>GGAKPLTDQEKRRQISIRGIVGVENVAELKKSFNRHLHFTLVKDRNVATTRDYYFALAHTVRDHLVGRWIRTQQHYYDKCPKRVYYLSLEFYMGRTLQNTMINLGLQNACDEAIYQLGLDIEELEEIEEDAGLGNGGLGRLAACFLDSMATLGLAAYGYGIRYEYGIFNQKIRDGWQVEEADDWLRYGNPWEKSRPEFMLPVHFYGKVEHTNTGTKWIDTQVVLALPYDTPVPGYMNNTVNTMRLWSARAPNDFNLRDFNVGDYIQAVLDRNLAENISRVLYPNDNFFEGKELRLKQEYFVVAATLQDIIRRFKASKFGSTRGAGTVFDAFPDQVAIQLNDTHPALAIPELMRIFVDIEKLPWSKAWELTQKTFAYTNHTVLPEALERWPVDLVEKLLPRHLEIIYEINQKHLDRIVALFPKDVDRLRRMSLIEEEGSKRINMAHLCIVGSHAVNGVAKIHSDIVKTKVFKDFSELEPDKFQNKTNGITPRRWLLLCNPGLAELIAEKIGEDYVKDLSQLTKLHSFLGDDVFLRELAKVKQENKLKFSQFLETEYKVKINPSSMFDVQVKRIHEYKRQLLNCLHVITMYNRIKKDPKKLFVPRTVIIGGKAAPGYHMAKMIIKLITSVADVVNNDPMVGSKLKVIFLENYRVSLAEKVIPATDLSEQ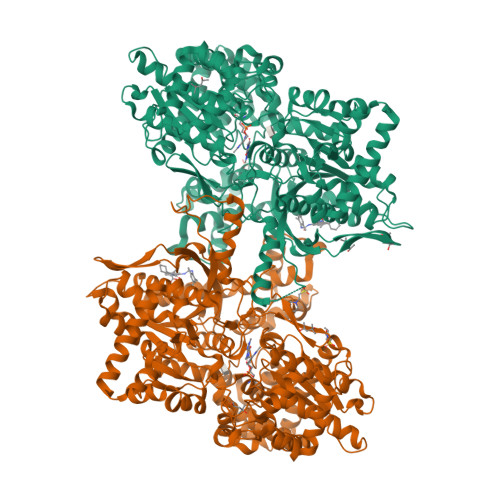ISTAGTEASGTGNMKFMLNGALTIGTMDGANVEMAEEAGEENLFIFGMRIDDVAALDKKGYEAKEYYEALPELKLVIDQIDNGFFSPKQPDLFKDIINMLFYHDRFKVFADYEAYVKCQDKVSQLYMNPKAWNTMVLKNIAASGKFSSDRTIKEYAQNIWNVEPSDLKISLSNESNKVNGN[2x]> ADVPAGVQLADKQTLVRNNGSEVQSLDPHKIEGVPESNVSRDLFEGLLISDVEGHPSPGVAEKWENKDFKVWTFHLRENAKWSDGTPVTAHDFVYSWQRLADPNTASPYASYLQYGHIANIDDIIAGKKPATDLGVKALDDHTFEVTLSEPVPYFYKLLVHPSVSPVPKSAVEKFGDKWTQPANIVTNGAYKLKNWVVNERIVLERNPQYWDNAKTVINQVTYLPISSEVTDVNRYRSGEIDMTYNNMPIELFQKLKKEIPNEVRVDPYLCTYYYEINNQKAPFNDVRVRTALKLALDRDIIVNKVKNQGDLPAYSYTPPYTDGAKLVEPEWFKWSQQKRNE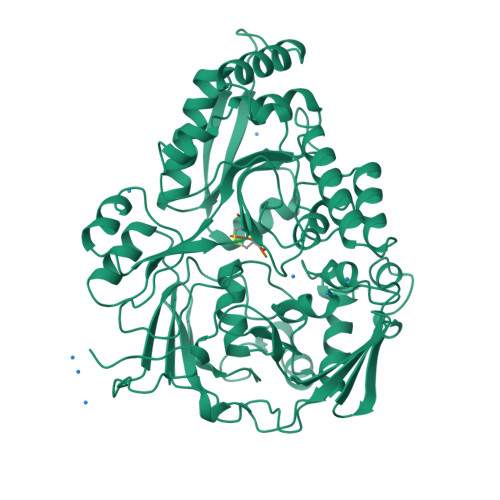EAKKLLAEAGFTADKPLTFDLLYNTSDLHKKLAIAVASIWKKNLGVNVNLENQEWKTFLDTRHQGTFDVARAGWCADYNEPTSFLNTMLSDSSNNTAHYKSPAFDKLIADTLKVADDTQRSELYAKAEQQLDKDSAIVPVYYYVNARLVKPWVGGYTGKDPLDNIYVKNLYIIKH;> KIK> GPLGSEDELYRQSLEIISRYLREQATGAKDTKPMGRSGATSRKALET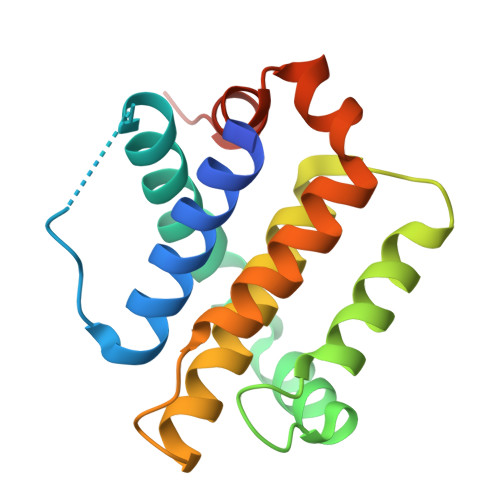LRRVGDGVQRNHETAFQGMLRKLDIKNEDDVKSLSRVMIHVFSDGVTNWGRIVTLISFGAFVAKHLKTINQESCIEPLAESITDVLVRTKRDWLVKQRGWDGFVEFFHVEDLEGG> MDEATWERMWKHVAKIHPDGEKVAQRIRGATDLPKIPIPSVPTFQPSTPVPERLEAVQRYIRELQYNHTGTQFFEIKKSRPLTGLMDLAKEMTKEALPIKALEAVILGIYLTNSMPTLERFPISFKTYFSGNYFRHIVLGVNFAGRYGALGMSRREDLMYKPPAFRTLSELVLDFEAAYGRCWHVLKKVKLGQ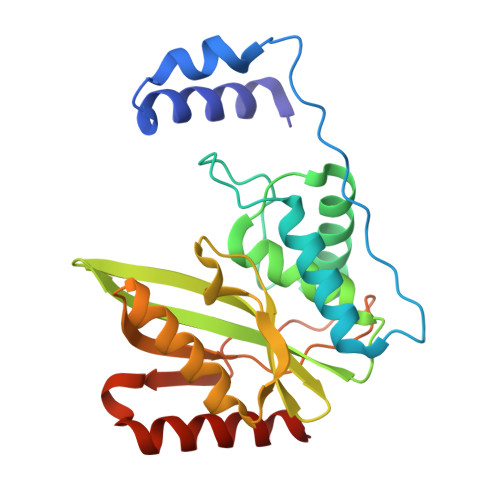SVSHDPHSVEQIEWKHSVLDVERLGRDDFRKELERHARDMRLKIG> GAMGDVSRLNQRNINELKIFVEKAKYYSIKLDAIYNECTGAYNDIMTYSEGTFSDQSKVNQAISIFKKDNKIVNKFKELEKIIEEYKPMFLSKLIDDFAIELDQAVDNDVSNARHVADSY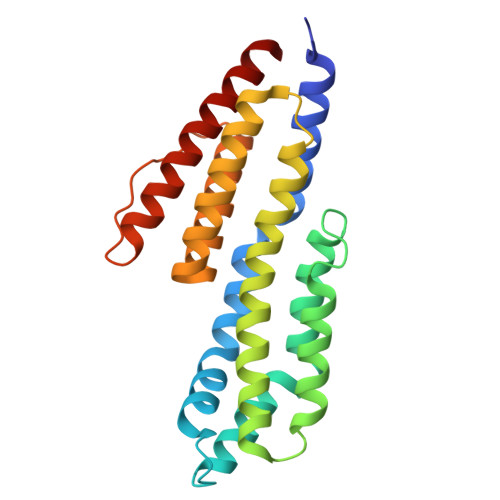KKLRKSVVLAYIESFDVISSKFVDSKFVEASKKFVNKAKEFVEENDLIALECIVKTIGDMVNDREINSRSRANNFAKKEADFLGAAVELEGAYKAIKQTLL> G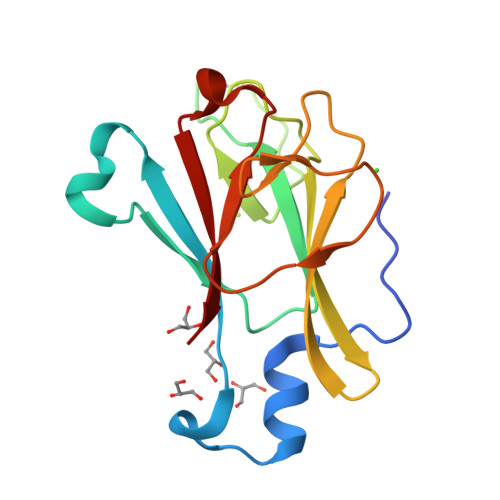AMGKHVEPQDAISPDNYMDMLGLEARDRTMYELVIYRKNDKDKGPWKRYDLNGRSCYLVGRELGHSLDTDLDDRTEIVVADIGIPEETSSKQHCVIQFRNVRGILKCYVMDLDSSNGTCLNNVVIPGARYIELRSGDVLTLSEFEEDNDYELIFMNV> EEE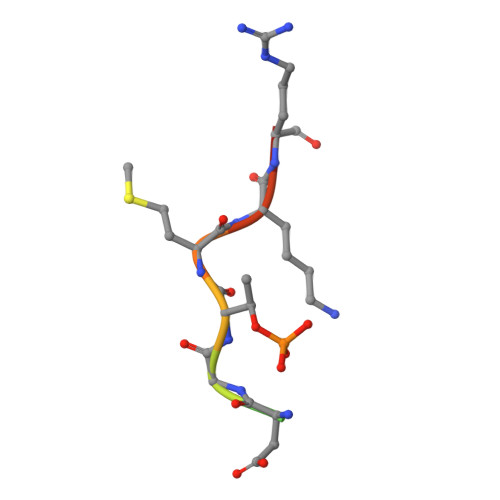DGTMKRN The nucleotide-activated sugar precursor UDP-glucose is produced from UTP and glucose-1-phosphate by UTP-glucose-1-phosphate uridylyltransferase (UGPase) enzymes. However, apart from GtaB, two other predicted UGPases, YtdA and YngB, are encoded in the B. subtilis 168 genome: as part of this study, we investigated the function of YngB. Here we show that, based on its crystal structure and in vitro and in vivo biochemical activity, the B. subtilis YngB protein is a functional UGPase. Furthermore, our data show that YngB is a functional UGPase that augments UDP-glucose production under oxygen-limiting conditions.

To determine the crystal structure of YngB, selenomethionine-substituted protein was produced in Escherichia coli and purified as a C-terminal His-tag fusion protein. The protein crystallized as a dimer in the asymmetric unit and the structure was solved at 2.80 Å by experimental phasing. YngB displayed a Rossmann fold with alternating α-helices and β-strands, which is commonly found in nucleotide-binding proteins. More specifically, the YngB monomer contains a central β-sheet surrounded by α-helices. Similar to the dimer interactions described for homologous UGPases, hydrogen bonds are formed between Tyr102 residues on the two β-strands located at the interface of the monomers, producing an extended central β-sheet spanning across the two subunits. The overall structure of YngB is very similar to homologous UGPases including A4JT02, GalUHp, and GalUCg as shown by superimposition. The outermost C-terminal α-helix is one of the most variable regions and absent either in GalUHp or in a different conformation in GalUCg. The structures superimposed with an RMSD of 1.61 Å and the putative UDP-glucose binding pocket could easily be identified in YngB. Based on this alignment, it can be predicted that residues Gly110, Gln105, Ala13, Gly14, Glu29, and Lys28 in YngB interact with the uridine moiety; Asp 133 is involved in the chelation of an Mg2+ ion; Asp 134, Val 204, Gly 172, and Glu 191 interact with the glucose moiety; and Lys 192 interacts with the diphosphate moiety. From these data, apparent Km values of 45.6 ± 3.24 μM (GtaB) and 42.1 ± 20.2 μM (YngB) were calculated for Glc-1-P and 49.5 ± 10.2 μM (GtaB) and 62.9 ± 13.8 μM (YngB) for UTP, respectively. kcat values of 1.06 s-1 (GtaB) and 0.264 s-1 (YngB) were calculated for Glc-1-P and 1.04 s-1 (GtaB) and 0.293 s-1 (YngB) for UTP, respectively.

>[2x]RKKVRKAVIPAAGLGTRFLPATKAQPKEMLPIVDKPAIQYIVEEAAESGIEDILIITGRNKRSIEDHFDRSAELEFNLREKGKTETLKEMQQIADLANIHYIRQKEPLGLGHAVLCAEHFIGDEPFAVLLGDDIMVSETPALRQLMDVYDVYGTEVVGVQSVLPEDVSKYGIINTSGSQGHVYEVNDLVEKPSPEEAPSEIAVMGRYVLNSSIFSVLKTIGRGAGNEIQLTDALREVCRKEPIHARLLEGNRYDIGDKLGCFKASTEIGLMRPEMRSQLLAYLEDVIKRETKEMLRL> MAMSNGNNDFVVLSNSSIATSAANPSPLTPCDGDHAAQQLTPKEATRTKVSPNGCLQLNGTVKSSFLPLDNQRMPQMLPQCCHPCPYHHPLTSHSSHQECHPEAGPAAPSALASCCMQPHSEYSASLCPNHSPVYQTTCCLQPS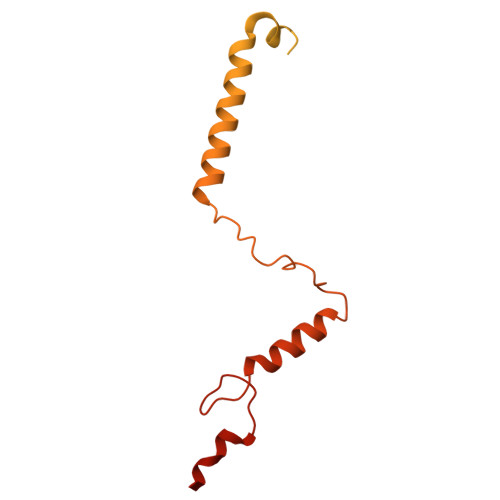PSFCLHHPWPDHFQHQPVQQHIANIRPSRPFKLPKSYAALIADWPVVVLGMCTMFIVVCALVGVLVPELPDFSDPLLGFEPRGTAIGQRLVTWNNMVKNTGYKATLANYPFKYADEQASSLEVLFQ methyl 4-[[3-[5-[2-(4-ethylsulfonylphenyl)ethanoylamino]thiophen-3-yl]pyridin-2-yl]oxymethyl]benzoate 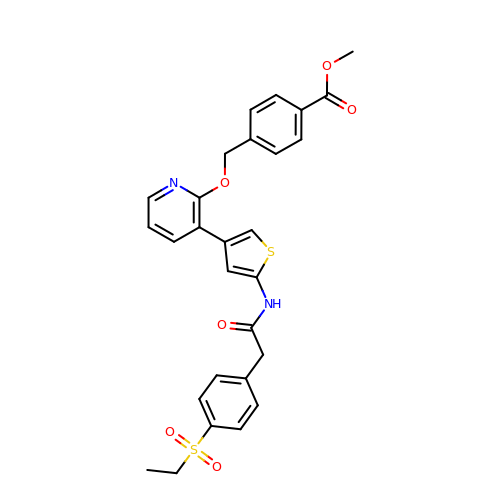| C28 H26 N2 O6 S2 | QOZJVJXEWQEQGR-UHFFFAOYSA-N>MGDKPIWEQIGSSFIQHYYQLFDNDRTQLGAIYIDASCLTWEGQQFQGKAAIVEKL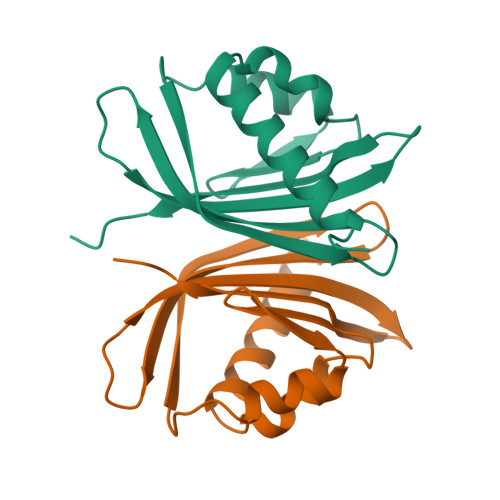SSLPFQKIQHSITAQDHQPTPDSCIISMVVGQLKADEDPIMGFHQMFLLKNINDAWVCTNDMFRLALHNFG[2x]> ENLYFQISRASGDAWDLADTIDDDDHRLVTCSPPTPIVSVAKLPNPEPIVTESLPEEDEEIVKSVIDGVIPSYSLESRLGDCKRAASIRREALQRVTGRSIEGLPLDGFDYESILGQCCEMPVGYIQIPVGIAGPLLLDGYEYSVPMATTEGCLVASTNRGCKAMFISGGATSTVLKDGMTRAPVVRFASARRASELKFFLENPENFDTLAVVFNRSSRFARLQSVKCTIAGKNAYVRFCCSTGDAMGMNMVSKGVQNVLEYLTDDFPDMDVIGISGNFCSDKKPAAVNWIEGRGKSVVCEAVIRGEIVNKVLKTSVAALVELNMLKNLAGSAVAGSLGGFNAHASNIVSAVFIATGQDPAQN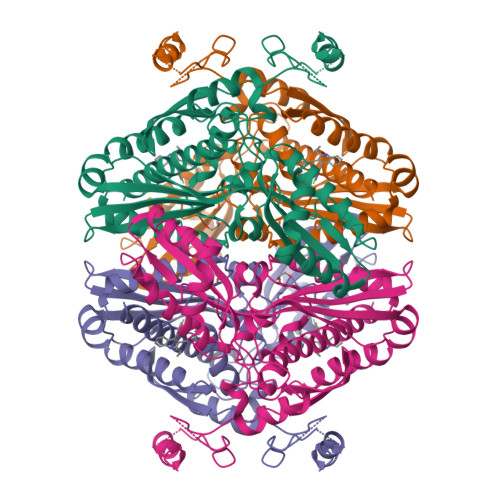VESSQCITMMEAINDGKDIHISVTMPSIEVGTVGGGTQLASQSACLNLLGVKGASTESPGMNARRLATIVAGAVLAGELSLMSAIAAGQLVRSHMKYNRSSRDISGATTTTTTTT Ral GTPases have been implicated as critical drivers of cell growth and metastasis in numerous Ras-driven cancers. Upon association with and activation by Ras·GTP, RalGDS activates the Ral (Ras-like) small GTPases, RalA, and RalB. The Ral GTPases share a panel of effectors including RLIP76 (also called RalBP1), members of the exocyst complex (Sec5 and Exo84), and the transcription factor ZONAB. Our solution structure of the RBD of RLIP76 in complex with RalB revealed that the interaction is mediated by a well-structured coiled-coil domain in which more than 80% of the interactions with Ral are mediated by the C-terminal α2 helix.

The tightest binding sequences, termed HLR (E427H/Q433L/K440R) and SMLR (E427S/L429M/Q433L/K440R), displayed affinities of 5 and 3 nM for RalA, respectively, a vast improvement on the wild-type RBD affinity of around 100 nM. We obtained high-quality crystals for both the RalB/RLIP76 RBD HLR and SMLR mutant complexes, which diffracted to 1.5 Å resolution. The HLR mutant increased the binding to RalB 28-fold, which is broadly similar to the improvements seen by SPA. A variant harboring the single Q433L mutation was produced and bound with a similar affinity to the HLR triple mutant, indicating that the Q433L mutation alone was sufficient to increase the affinity for RalB by 25-fold. The mutant RBD structures show that the side chain of Leu433 contributes to a hydrophobic network of interactions involving several Ral residues (Ala48, Leu67, Tyr82) and Trp430 of RLIP76. In the wild-type RBD complex, Gln433 points out to the solvent, leaving a space at the edge of the hydrophobic pocket where Trp430 is buried in an interaction known to be essential for the binding affinity. When the Gln is replaced by Leu, the side chain shifts toward the pocket and fills this space. Replacement with arginine in the HLR and SMLR mutants allows this hydrogen bond to be maintained while an additional hydrogen bond with the backbone carbonyl of RalB Ala48 is gained. However, the K440R mutation only exerts a minimal improvement in binding of the RBD to Ral proteins, as evidenced by comparison of the E427H/Q433L (HL) double mutant with the E427H/Q433L/K440R (HLR) triple mutant, which bind with similar affinities. The replacement of Glu427 with histidine or serine breaks a salt bridge formed with RalB without forming any new interactions and ITC data demonstrated that this substitution did not improve binding to Ral proteins.

>[2x]MAANKSKGQSSLALHKVIMVGSGGVGKSALTLQFMYDEFVEDYEPTKADSYRKKVVLDGEEVQIDILDTAGLEDYAAIRDNYFRSGEGFLLVFSITEHESFTATAEFREQILRVKAEEDKIPLLVVGNKSDLEERRQVPVEEARSKAEEWGVQYVETSAKTRANVDKVFFDLMREIRTKKMSENK;>GPLGSETQAGIKEEIRRQEFLLNSLHRDLQGGIKDLSKEHRLWEVLRILTALRRKLREA[2x]>[4x]GSHMKFTVEREHLLKPLQQVSGPLGGRPTLPILGNLLLQVADGTLSLTGTDLEMEMVARVALVQPHEPGATTVPARKFFDICRGLPEGAEIAVQLEGERMLVRSGRSRFSLSTLPAADFPNLDDWQSEVEFTLPQATMKRLIEATQFSMAHQDVRYYLNGMLF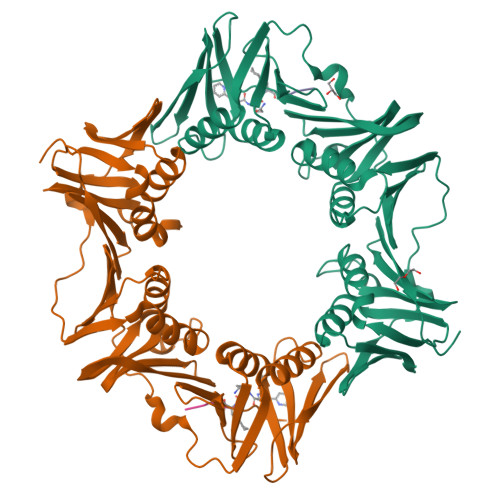ETEGEELRTVATDGHRLAVCSMPIGQSLPSHSVIVPRKGVIELMRMLDGGDNPLRVQIGSNNIRAHVGDFIFTSKLVDGRFPDYRRVLPKNPDKHLEAGCDLLKQAFARAAILSNEKFRGVRLYVSENQLKITANNPEQEEAEEILDVTYSGAEMEIGFNVSYVLDVLNALKCENVRMMLTDSVSSVQIEDAASQSAAYVVMPMRL;>[4x]XQADLF>GANMAGRSMQAARCPTDELSLSNCAVVSEKDYQSGQHVIVRTSPNHKYIFTLRTHPSVVPGSVAFSLPQRKWAGLSIGQEIEVALYSFDKAKQCIGTMTIEIDFLQKKNIDSNPYDTDKMAAEFIQQFNNQAFSVGQQLVFSFNDKLFGLLVKDIEAMDPSILKGEPASGKRQKIEVGLVVGNSQVAFEKAENSSLNLIGKAKTKENRQSIINPDWNFEKMGIGGLDKEFSDIFRRAFASRVFPPEIVEQMGCKHVKGILLYGPPGCGKTLLARQIGKMLNAREPKVVNGPEILNKYVGESEANIRKLFADAEEEQRRLGANSGLHIIIFDEIDAICKQRGSMAGSTGVHDTVVNQLLSKIDGVEQLNNILVIGMTNRPDLIDEALLRPGRLEVKMEIGLPDEKGRLQILHIHTARMRGHQLLSADVDIKELAVETKNFSGAELEGLVRAAQSTAMNRHIKASTKVEVDMEKAESLQVTRGDFLASLENDIKPAFGTNQEDYASYIMNGIIKWGDPVTRVLDDGELLVQQTKNSDRTPLVSVLLEGPPHSGKTALAAKIAEESNFPFIKICSPDKMIGFSETAKCQAMKKIFDDAYKSQLSCVVVDDIERLLDYVPIGPRFSNLVLQALLVLLKKAPPQGRKLLIIGTTSRKDVLQEMEMLNAFSTTIHVPNIATGEQLLEALELLGNFKDKERTTIAQQVKGKKVWIGIKKLLMLIEMSLQMDPEYRVRKFLALLREEGASPLDFD[6x];>[2x]MKDRTQELRTAKDSDDDDDVTVTVDRDRFMDEFFEQVEEIRGFIDKIAENVEEVKRKHSAILASPNPDEKTKEELEELMSDIKKTANKVRSKLKSIEQSIEQEEGLNRSSADLRIRKTQHSTLSRKFVEVMSEYNATQSDYRERCKGRIQRQLEITGRTTTSEELEDMLESGNPAIFASGIIMDSSISKQALSEIETRHSEIIKLENSIRELHDMFMDMAMLVESQGEMIDRIEYNVEHAVDYVERAVSDTKKAVKYQSKARRKKIM;>MGSSHHHHHHSQDPNSMAEDADMRNELEEMQRRADQLADESLESTRRMLQLVEESKDAGIRTLVMLDEQGEQLERIEEGMDQINKDMKEAEKNLTDLGKFAGLAVAPANKLKSSDAYKKAWGNNQDGVVASQPARVVDEREQMAISGGFIRRVTNDARENEMDENLEQVSGIIGNLRHMALDMGNEIDTQNRQIDRIMEKADSNKTRIDEANQRATKMLGSG[2x];>[4x]GMDTSGKQAEAMALLAEAERKVKNSQSFFSGLFGGSSKIEEACEIYARAANMFKMAKNWSAAGNAFCQAAQLHLQLQSKHDAATCFVDAGNAFKKADPQEAINCLMRAIEIYTDMGRFTIAAKHHISIAEIYETELVDVEKAIAHYEQSADYYKGEESNSSANKCLLKVAGYAAQLEQYQKAIDIYEQVGTSAMDSPLLKYSAKDYFFKAALCHFCIDMLNAKLAVQKYEELFPAFSDSRECKLMKKLLEAHEEQNVDSYTESVKEYDSISRLDQWLTTMLLRIKKTIQGDEEDLR

The membrane-anchored SNARE (soluble N-ethylmaleimide-sensitive factor acceptor protein receptor) proteins provide the energy to drive membrane fusion in various cellular contexts, such as intracellular trafficking and exocytosis. Supercomplexes of NSF, α-SNAP, and either a syntaxin tetramer or one of two binary complexes of syntaxin—SNAP-25 reveal atomic details of SNARE processing and show how sequential ATP hydrolysis drives disassembly. NSF comprises three structured domains connected by flexible linkers—the adapter N-domain followed by the D1 and D2 AAA+ domains. Six NSF protomers come together to form the active form of the enzyme, a homo-hexamer.

A representative 22bin20S model (class #19, 3.56 Å) and ɑ-SNAP—2:2 binary SNARE subcomplex model (class #23, 4.14 Å). A Hexameric NSF engages the ɑ-SNAP—2:2 binary SNARE subcomplex via N-domains (salmon), which engage three ɑ-SNAP molecules (gold) surrounding the soluble, 2:2 binary SNARE complex composed of two syntaxin H3 domains (dark red) and two SNAP-25 SN1 domains contributed by two separate full-length SNAP-25 molecules (green). A portion of a linker N-terminal to one syntaxin H3 domain is observed within the catalytic D1 ring of NSF (light blue). The D2 ring of NSF (purple) shows no substrate density. B NSF (light blue) engages one of the two syntaxin molecules (dark red) in the 2:2 binary SNARE complex via pore loop interactions involving Y294 (protomers A–F, indicated). Of the five 22bin20S classes with the 2:2 binary SNARE complex, all are found with syntaxin in the D1 pore, while two are observed with the N-terminus of the SNAP-25 SN1 domain in the pore. Substrate-bound reconstructions reveal a flattened D1 ring in closer proximity to the D2 ring and a strikingly different ɑ-SNAP—SNARE spire structure than observed in the 21bin20S complex under non-hydrolyzing conditions. Even without further processing, this structure was recognizable as a parallel 2:2 syntaxin—SNAP-25 sub-complex formed by two syntaxin H3 SNARE domains and two SNAP-25 SN1 SNARE domains; this binary 2:2 configuration was previously observed in crystal structures of syntaxin-1 H3 and SNAP-25 SN1 domains and was unexpected as we prepared the complex with full-length proteins, implying that two independent SNAP-25 molecules contribute their SN1 SNARE domains to this complex. Unlike the non-hydrolyzing 21bin20S reconstructions, hydrolyzing 22bin20S reconstructions are only ATP+Mg2+-bound and substrate engaged in protomer E, consistent with a sequential hydrolysis mechanism (middle column). Except for the rebinding F protomer described above, all other D1 protomers are ADP bound with variability in the presence of Mg2+ and inorganic phosphate (Pi); in most cases, protomers C and D have ADP•Pi and Mg2+, protomer B is usually ADP-bound, and protomer A is always ADP-bound.(2S)-2-(4-aminophenyl)-1-hydroxy-5-methoxy-1,2-dihydro-3H-indol-3-one | C15 H12 N2 O3 | 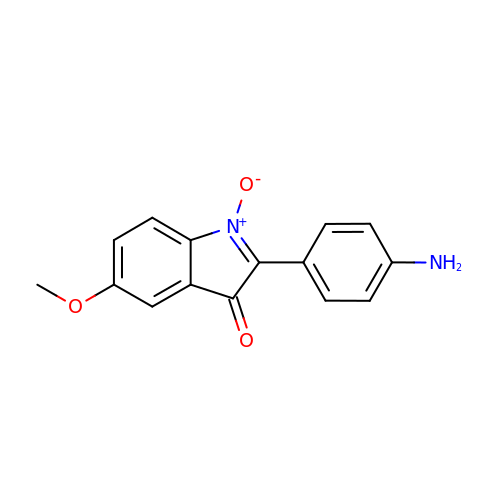HTBDGBPUYWVYCA-UHFFFAOYSA-N> MRESAAQKFQRQHMDPDGSSINSPTYCNQMMKRRDMTNGSCKPVNTFVHEPLADVQAVCSQENVTCKNRKSNCYKSSSALHITDCHLKGNSKYPNCDYK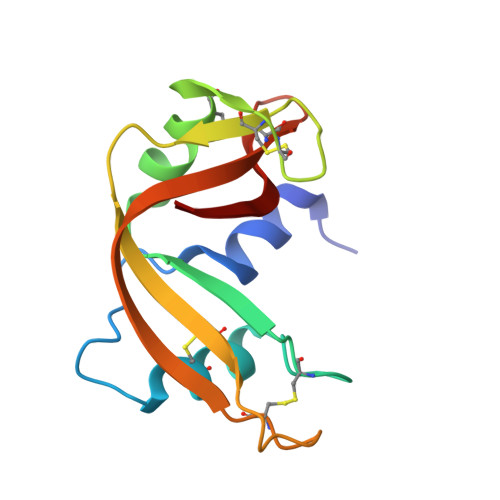TTQYQKHIIVACEGNPYVPVHFDATV>[2x]MDYRQLHRWDLPPEEAIKVQNELRKKIKLTPYEGEPEYVAGVDLSF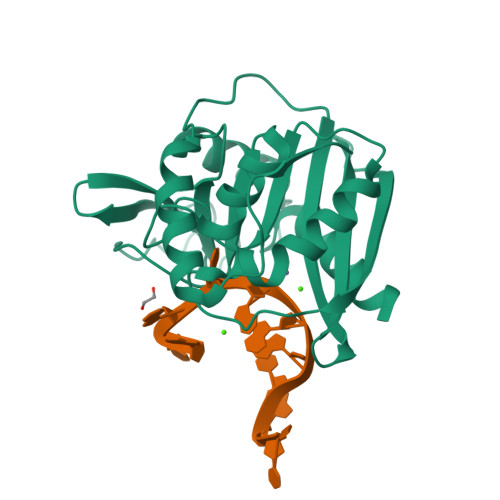PGKEEGLAVIVVLEYPSFKILEVVSERGEITFPYIPGLLAFREGPLFLKAWEKLRTKPDVVVFNGQGLAHPRKLGIASHMGLFIEIPTIGVAKSRLYGTFKMPEDKRCSWSYLYDGEEIIGCVIRTKEGSAPIFVSPGHLMDVESSKRLIKAFTLPGRRIPEPTRLAHIYTQRLKKGLF> QILSIDPLDISQNLAAVNKSLSDALQHLA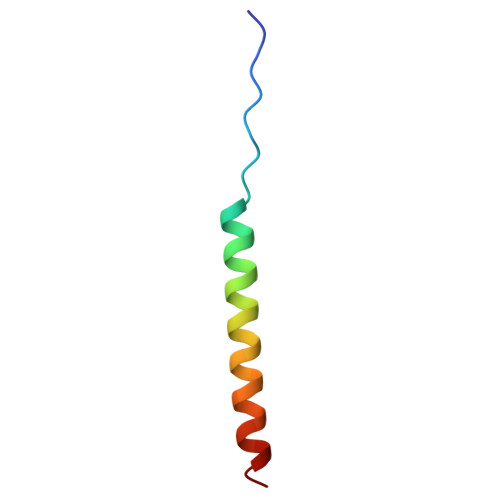QSDTYLSAI>[2x]GIDPFTGIDPFTKFFYSDQNVDSRDPVQLNLLYVQARDDILNGSHPVSFEKACEFGGFQAQIQFGPHVEHKHKPGFLDLKEFLPKEYIKQRGAEKRIFQEHKNCGEMSEIEAKVKYVKLARSLRTYGVSFFLVKEKMKGKNKLVPRLLGITKDSVMRVDEKTKEVL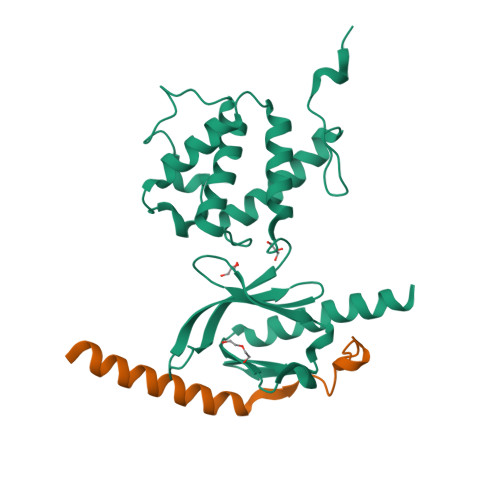QEWPLTTVKRWAASPKSFTLDFGEYQESYYSVQTTEGEQISQLIAGYIDIILKKKQS;>GPKLLMIIHDRREFAKFEKEKMNAKWDTQENPIYKSPINNFKNPNYGRKAGL[2x]>[2x]STTLTRQDLNFGQVVADVLCEFLEVAV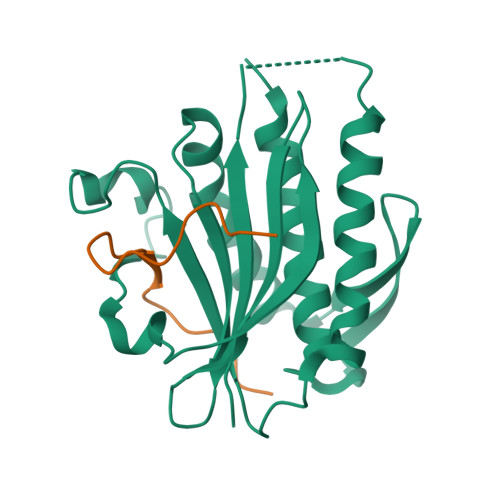HLILYVREVYPVGIFQKRKKYNVPVQMSCHPELNQYIQDTLHCVKPLLEKNDVEKVVVVILDKEHRPVEKFVFEITQPPLLSISSDSLLSHVEQLLAAFILKISVCDAVLDHNPPGCTFTVLVHTREAATRNMEKIQVIKDFPWILADEQDVHMHDPRLIPLKTMTSDILKMQLYVEERAHKGS;>[2x]MLSRFIPWFPYDGSKLPLRPKRSPPASREEIMATL>MPGSLIDTRQQPLSVGIVGGGIIGVILAAGLVRRGIDVKVFEQARGFREIGAGMAFTANAVRCMEMLDPAIVWALRSSGAVPISIGDHQAEARDYLRWVDGYHESSKRLYQLDAGIRGFEACRRDQFLEALVKVLPEGIVECQKRLQKIHEKNETEKVTLEFADGTFAHVDCVIGADGIRSRVRQHLFGEDSPYSHPHYSHKFAFRGLITMENAISALGEDKARTLNMHVGPNAHLIHFPVANETMVNIAAFVSDPEEWPDKLSL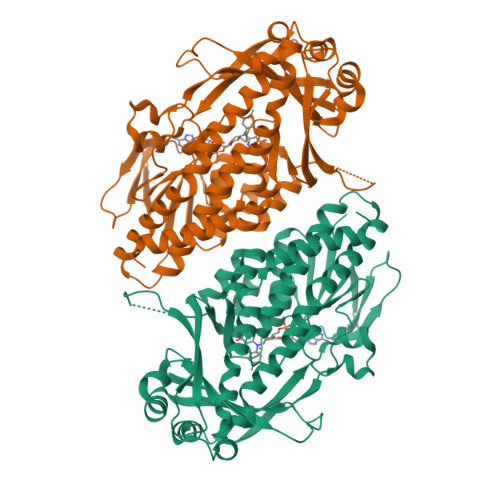VGPATREEAMGYFANWNPGLRAVLGFMPENIDRWAMFDTYDYPAPFFSRGKICLVGDAAHAAVPHHGAGACIGIEDALCATVLLAEVFVSTRGKSSIVRNRAIAAAFGSFNAVRRVRAQWFVDSSRRVCDLYQQPEWADPQKRIKAENCFEEIKDRSHKIWHFDYNSMLQEAIEKYRHNMGS[2x]> MGSSHHHHHHSSGPQQGLRQAQTPQDRIHYTGKELSNPTYHDGQLSPVVGVHNIQLVRANREHPEASNGNGWTYNHQPMLAYWNGQFYYQYLADPSDEHVPPSQTFLMTSKDGYQWTNPEIVFPPYKVPDGYTKESRPGMQAKDLIAIMHQRVGFYVSKSGRLITMGNYGVALDKKDDPNDGNGIGRVVREIKKDGSFGPIYFIYYNHGFNEKNTDYPYFKKS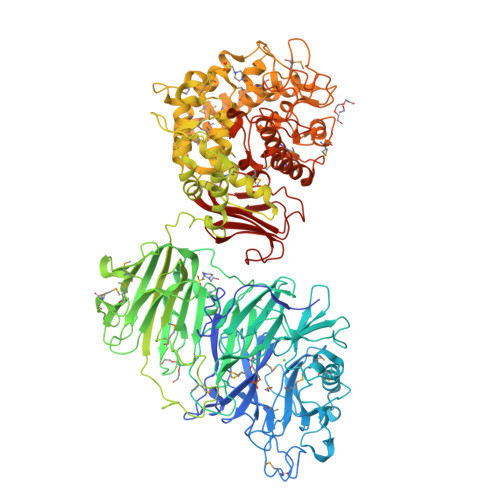KDREFVKACQEILDNPLYMMQWVEEADREDPIIPLKKGYKAFNCYTLPDGRIASLWKHALTSISEDGGHTWAEPVLRAKGFVNSNAKIWGQRLSDGTYATVYNPSEFRWPLAISLSKDGLEYTTLNLVHGEITPMRYGGNYKSYGPQYPRGIQEGNGVPADGDLWVSYSVNKEDMWISRIPVPVQINASAHADDDFSKSGSIAELTNWNIYSPVWAPVSLEGEWLKLQDKDPFDYAKVERKIPASKELKVSFDLSAGQNDKGILQIDFLDENSIACSRLELTPDGIFRMKGGSRFANMMNYEAGKTYHVEAVLSTADRNIQVYVDGKRVGLRMFYAPVATIERIVFRTGEMRTFPTVDTPADQTYDLPDAGGQEPLAEYRIANVKTSSTDKDASSAFLKYADFSHYAESFNGMEDENIVQAIPNAKASEWMEENIPLFECPQRNFEEMYYYRWWSLRKHIKETPVGYGMTEFLVQRSYSDKYNLIACAIGHHIYESRWLRDPKYLDQIIHTWYRGNDGGPMKKMDKFSSWNADAVLARYMVDGDKDFMLDMTKDLETEYQRWERTNRLKNGLYWQGDVQDGMEESISGGRNKKYARPTINSYMYGNAKALSIMGILSGDEGMAMRYGMRADTLKSLVENDLWNTRHQFFETMRTDSSANVREAIGYIPWYFNLPDTTKKYEVAWKEIMDEKGFSAPYGLTTAERRHPEFRTRGVGKCEWDGAIWPFASAQTLTAMANFMNNYPQTVLSDSVYFRQMELYVESQYHRGRPYIGEYLDEVTGYWLKGDQERSRYYNHSTFNDLMITGLIGLRPRLDDTIEINPLIPADKWDWFCLDNVLYHGHNLTILWDKNGDRYHCGKGLRIFVNGKEAGHADTLTRLVCENALK> GSSGSSGMQIGKIIKVSGPLVMAENMSEACIQDMCLVGDLGVIGEIIEMRQDVASIQVYEETSGIGPGEPVRSTGEALSVELGPGIISQMFDGIQRPLDTFMEVTQSNFLGRGVQLPALDHEKQWWFEATIEEGTEVSAGDIIGYVDETKIIQHKIMVPNGIKGTVQKIESGSFTIDDPICVIETEQGLKELTMMQKWPVRRGRPIKQKLNPDVPMITGQRVIDTFFPVTKGGAAAVPGPFGAGKTVVQHQIAKWSDVDLVVYVGCGERGNEMTDVVNEFPELIDPNTGESLMERTVLIANTSNMPVAAREASIYTGITIAEYFRDMGYDVAIMADSTSRWAEALREMSGRLEEMPGDEGYPAYLGSRLAEYYERSGRVIALGSDQREGSITAISAVSPSGGDISEPVTQNTLRVVKVFWGLDSSLAQKRHFPSINWIQSYSLYSTEVGRYMDQILQQDWSDMVTEGMRILQEEEQLNEIVRLVGIDSLSDNDRLTLEVAKSIRED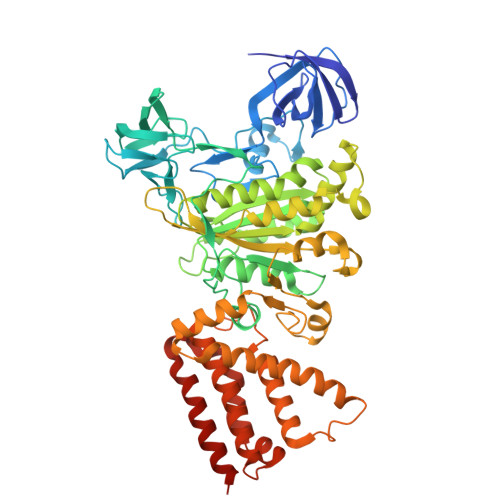YLQQNAFDDVDTFTSREKQFNMLKVILTFGKEARKALSLGAYFNEIMEGTVAVRERISRSKYIPEEELAKISSINEEIKETIQLIVSEGGMTDD> GHMGAPAPVVVCYPGGAVNERDADQAMDAMLRVVERVGQWPEKSFSSVFTAKVADCGKLMAEMKPAFAITSLALYLDMRGQYDLVPVVQPRIDGRTSERYRVVAKQGRFHDMDELKGRTLGGTMLDEPAFLGKIVFAGKYDPEKDFALQPSRQ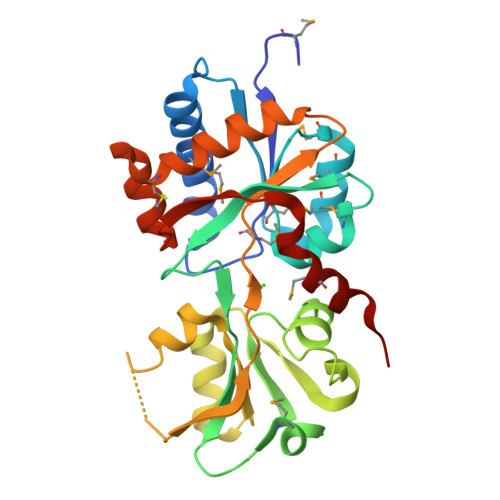AIRALRSLDKGELDAVVLNEQQFAGLSALQLASPVETVFTSAEIPLMGVVANARLTSAQERARFAQALETLCADPEGRKLCDLFGIQSFVAVDPTVFDPMARLWLARN> MSMAMSQSNRELVVDF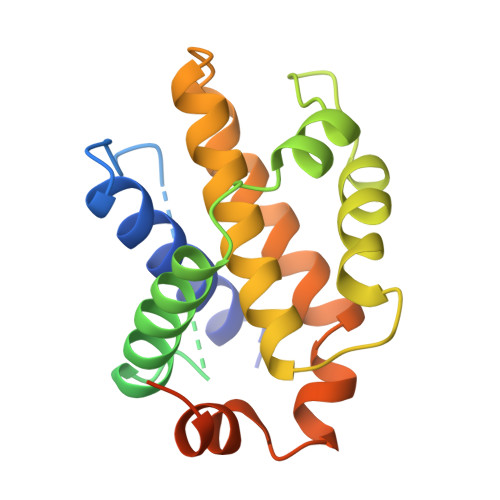LSYKLSQKGYSWSQFSDVEENRTEAPEGTESEMETPSAINGNPSWHLADSPAVNGATGHSSSLDAREVIPMAAVKQALREAGDEFELRYRRAFSDLTSQLHITPGTAYQSFEQVVNELFRDGVNWGRIVAFFSFGGALCVESVDKEMQVLVSRIAAWMATYLNDHLEPWIQENGGWDTFVELYGNNAAAESRKGQERLEHHHHHH> GPGLKQKIVIKVAMEGNNCRSKAMALVASTGGVDSVALVGDLRDKIEVVGYGIDPIKLI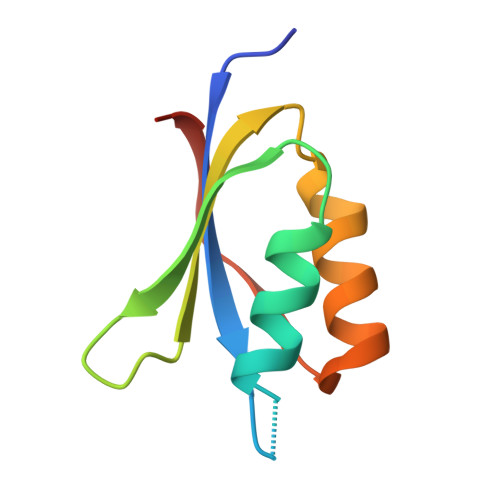SALRKKVGDAELLQVSQAKED> DGSLQLELGTFNLHTLFREVLNLIKPIAVVKKLPITLNLAPDLPEFVVGDEKRLMQIILNIVGNAVKFSKQGSISVTALVTKSDTRAADFFVVPTGSHFYLRVKVKDSGAGINPQDIPKIFT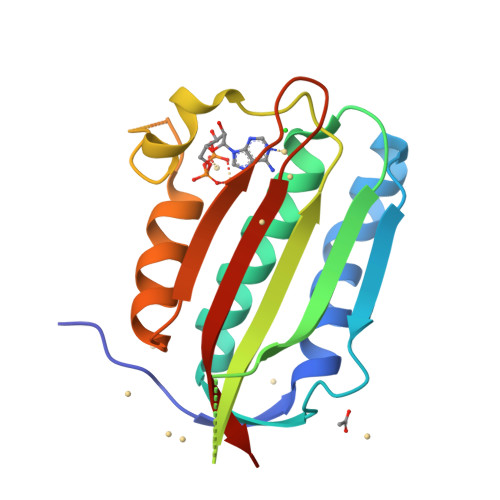KFAQTQSLATRSSGGSGLGLAISKRFVNLMEGNIWIESDGLGKGCTAIFDVKLGISERSNE N-[(1,3-dimethyl-1H-pyrazol-5-yl)methyl]-5-methyl-3H-imidazo[4,5-b]pyridin-2-amine 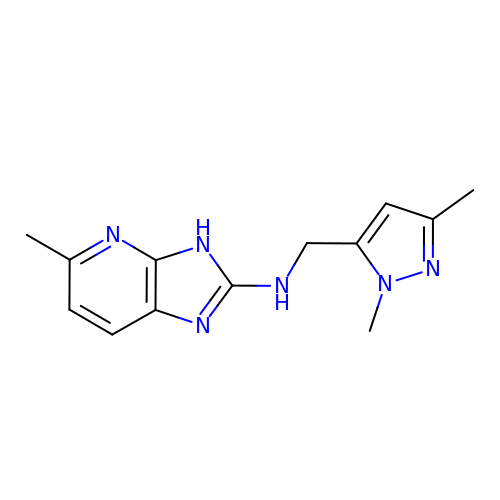| C13 H16 N6 | CZOWPFJOPIQOCT-UHFFFAOYSA-N S-[2-[3-[[(2R)-4-[[[(2R,3S,4R,5R)-5-(6-aminopurin-9-yl)-4-hydroxy-3-phosphonooxy-oxolan-2-yl]methoxy-hydroxy-phosphoryl]oxy-hydroxy-phosphoryl]oxy-2-hydroxy-3,3-dimethyl-butanoyl]amino]propanoylamino]ethyl] (2R)-2-hydroxy-4-methyl-pentanethioate | C27 H46 N7 O18 P3 S | 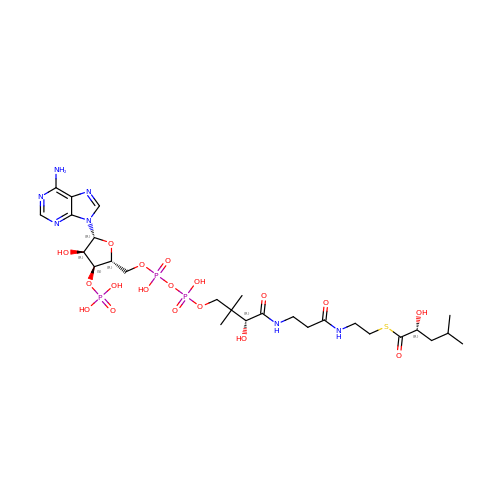CFNPCSNXESBNGR-LYALRYAQSA-N>[3x]AEIDEGVFETTATIDNGSFGTRTIRFETGRLALQAAGAVVAYLDDDNMLLSATTASKNPKEHFDFFPLTVDVEERMYAAGRIPGSFFRREGRPSTDAILTCRLIDRPLRPSFVDGLRNEIQIVVTILSLDPGDLYDVLAINAASASTQLGGLPFSGPIGGVRVALIDGTWVGFPTVDQIERAVFDMVVAGRIVEGDVAIMMVEAEATENVVELVEGGAQAPTESVVAAGLEAAKPFIAALCTAQQELADAAGKSGKPTVDFPVFPDYGEDVYYSVSSVATDELAAALTIGGKAERDQRIDEIKTQVVQRLADTYEGREKEVGAALRALTKKLVRQRILTDHFRIDGRGITDIRALSAEVAVVPRAHGSALFERGETQILGVTTLDMIKMAQQIDSLGPETSKRYMHHYNFPPFSTGET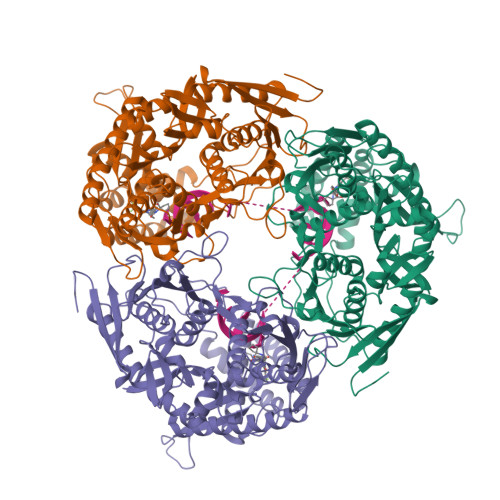GRVGSPKRREIGHGALAERALVPVLPSVEEFPYAIRQVSEALGSNGSTSMGSVCASTLALLNAGVPLKAPVAGIAMGLVSDDIQVEGAVDGVVERRFVTLTDILGAEDAFGDMDFKVAGTKDFVTALQLDTKLDGIPSQVLAGALEQAKDARLTILEVMAEAIDRPDEMSPYAPR>XDYLRELLKLELQLIKQYREALEYVKLPVLAK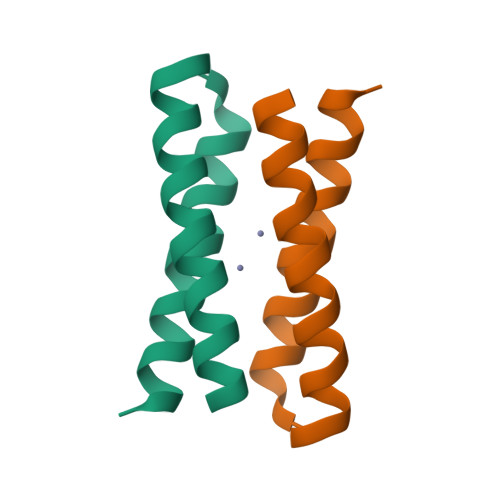ILEDEEKHIEWLETILGX[3x]>GSHMMNDGKQQSTFLFHDYETFGTHPALDRPAQFAAIRTDSEFNVIGEPEVFYCKPADDYLPQPGAVLITGITPQEARAKGENEAAFAARIHSLFTVPKTCILGYNNVRFDDEVTRNIFYRNFYDPYAWSWQHDNSRWDLLDVMRACYALRPEGINWPENDDGLPSFRLEHLTKANGIEHSNAHDAMADVYATIAMAKLVKTRQPRLFDYLFTHRNKHKLMALIDVPQMKPLVHVSGMFGAWRGNTSWVAPLAWHPENRNAVIMVDLAGDISPLLELDSDTLRERLYTAKTDLGDNAAVPVKLVHINKCPVLAQANTLRPEDADRLGINRQHCLDNLKILRENPQVREKVVAIFAEAEPFTPSDNVDAQLYNGFFSDADRAAMKIVLETEPRNLPALDITFVDKRIEKLLFNYRARNFPGTLDYAEQQRWLEHRRQVFTPEFLQGYADEL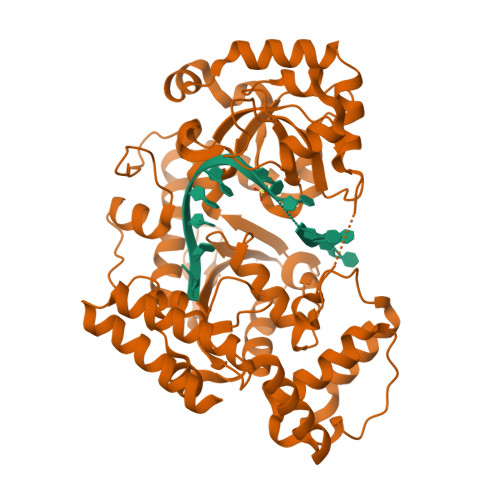QMLVQQYADDKEKVALLKALWQYAEEIV[2x]>AMKKDSKAPCVEVFDERDGCKAAGTQKASGDDGFCVKVSMKAIGFNAAEAASVTKNYGIKRFGAKSV[2x];>[2x]MLDAFSKVITSADGKAAYVGGADLQALKKFVSEGNKRMDSVNAIVSNASCIVSDSVSGMVCENPSLIAPNGGVYTN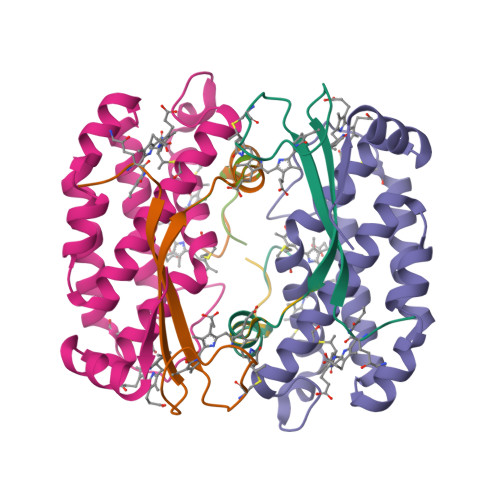RKMAACLRDAEIILRYVSYSLLSGDSSVLEDRCLNGLKETYASLGVPAAGNARTISIMKATVIGFITNNSQQKKLSTPAGDCSALASEVGGYFDKVSSALA;>AMKKDSKAPCVEVFDERDGCKAAGTQKASGDDGFCVKVSMKAIKMNAAEATSVTKNYNTKLL[2x]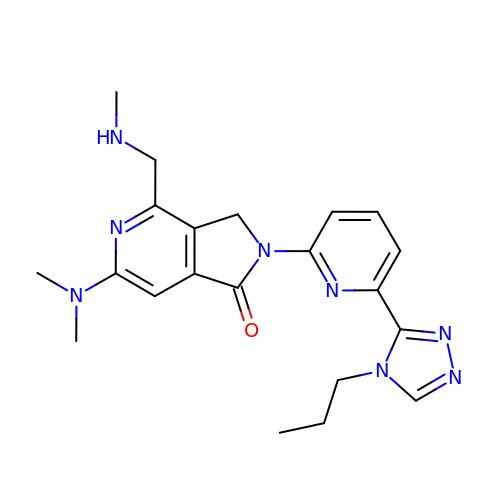6-(dimethylamino)-4-[(methylamino)methyl]-2-[6-(4-propyl-4H-1,2,4-triazol-3-yl)pyridin-2-yl]-2,3-dihydro-1H-pyrrolo[3,4-c]pyridin-1-one | C21 H26 N8 O | XVKPIWUWUZOHIR-UHFFFAOYSA-N(1~{R},2~{S},3~{S},4~{S},5~{R},6~{R})-5-azanyl-6-(hydroxymethyl)cyclohexane-1,2,3,4-tetrol | C7 H16 N O5 | 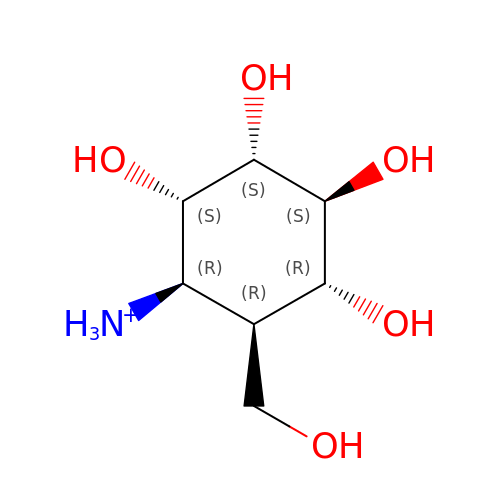SWVTZDDSAFUTKS-ARYBSUEZSA-O>MDQETVGNVVLLAIVTLISVVQNGFFAHKVEHESRTQNGRSFQRTGTLAFERVYTANQNCVDAYPTFLAVLWSAGLLCSQVPAAFAGLMYLFVRQKYFVGYLGERTQSTPGYIFGKRIIL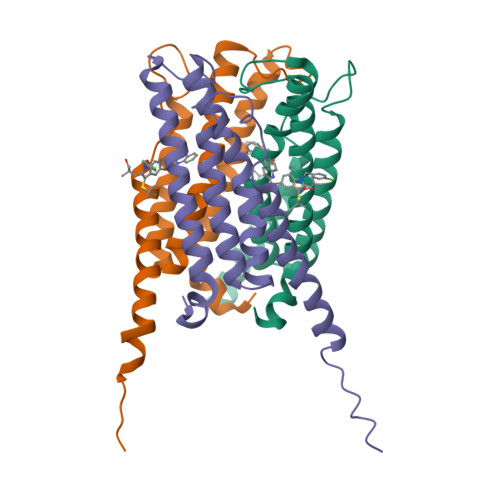FLFLMSVAGIFNYYLIFFFGSDFENYIATISTTISPLLLIP[6x]>XSKLLELLRKLAEALHKAIELLEKWG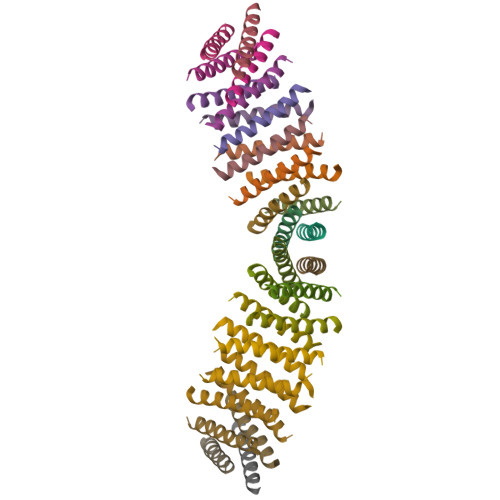X[16x]β-d-Glucosidases (EC 3.2.1.21) are classical glycoside hydrolases that catalyse the hydrolysis of the nonreducing terminal glucose from β-linked d-gluco-oligosaccharides and aryl-β-d-glucosides. Here, the three-dimensional structures of two industrially important family GH3 β-d-glucosidases from Aspergillus fumigatus and A. oryzae, solved by molecular replacement and refined at 1.95 Å resolution, are reported. Both enzymes, which share 78% sequence identity, display a three-domain structure with the catalytic domain at the interface, as originally shown for barley β-d-glucan exohydrolase, the first three-dimensional structure solved from glycoside hydrolase family GH3.

In AoβG the four protomers in the asymmetric unit are arranged as two dimers, with the second (chains C and D) at right angles to the first (chains A and B), interacting via their FnIII domains (chain A with C and chain B with D). There are no sugar-mediated interactions in the FnIII dimer–dimer interfaces, which are comprised solely of protein–protein and protein–solvent hydrogen bonds, whilst there are a couple of interactions between glycans at the subunit–subunit interface between chains A and B and chains C and D within each dimer, as detailed below. In AoβG there is a PEG molecule bound in the +1 site, hydrogen-bonded to Asp93 OD2 (in three of the four molecules) and/or to Arg99 NH1 (in two of the four protomers in the asymmetric unit). Substrate-specificity studies with AoβG have demonstrated a tight specificity for β-d-glucopyranoside in the −1 subsite, with a much broader tolerance at the +1 subsite with similar catalytic efficiencies for glucose-β-1,2-, β-1,3-, β-1,4- and β-1,6-linked glucose and p-nitrophenyl-β-d-glucopyranoside. There are 13 potential N-glycosylation sites in the amino-acid sequences of each of AfβG and AoβG, with nine and ten of them being occupied in their respective crystal structures; we have modelled 45 and 46 sugars in chains A and B, respectively, for AfβG, whilst AoβG has 40, 42, 41 and 34 sugars modelled in chains A, B, C and D, respectively. The largest N-glycan is linked to Asn323 in domain A, where it is visible as a complete nine-mannose tree in AfβG and AoβG (chains A and B in the latter, chains C and D having seven and six mannoses, respectively). Intriguingly, those sites located on the protein surface (Asn543 and Asn715 in AfβG, Asn212 and Asn543 in AoβG) appear to have been truncated to a single GlcNAc molecule linked to their corresponding Asn residue, despite no attempt having been made to remove external N-glycans enzymatically. In addition, the external site at Asn713 in AoβG (equivalent to Asn715 in AfβG) remained uncleaved even though the first GlcNAc molecule is in a very similar position and orientation to its equivalents in the other two structures.

>[4x]KDDLAYSPPFYPSPWADGQGEWAEVYKRAVDIVSQMTLTEKVNLTTGTGWQLERCVGQTGSVPRLNIPSLCLQDSPLGIRFSDYNSAFPAGVNVAATWDKTLAYLRGQAMGEEFSDKGIDVQLGPAAGPLGAHPDGGRNWEGFSPDPALTGVLFAETIKGIQDAGVIATAKHYIMNEQEHFRQQPEAAGYGFNVSDSLSSNVDDKTMHELYLWPFADAVRAGVGAVMCSYNQINNSYGCENSETLNKLLKAELGFQGFVMSDWTAHHSGVGAALAGLDMSMPGDVTFDSGTSFWGANLTVGVLNGTIPQWRVDDMAVRIMAAYYKVGRDTKYTPPNFSSWTRDEYGFAHNHVSEGAYERVNEFVDVQRDHADLIRRIGAQSTVLLKNKGALPLSRKEKLVALLGEDAGSNSWGANGCDDRGCDNGTLAMAWGSGTANFPYLVTPEQAIQNEVLQGRGNVFAVTDSWALDKIAAAARQASVSLVFVNSDSGEGYLSVDGNEGDRNNITLWKNGDNVVKTAANNCNNTVVIIHSVGPVLIDEWYDHPNVTGILWAGLPGQESGNSIADVLYGRVNPGAKSPFTWGKTRESYGSPLVKDANNGNGAPQSDFTQGVFIDYRHFDKFNETPIYEFGYGLSYTTFELSDLHVQPLNASRYTPTSGMTEAAKNFGEIGDASEYVYPEGLERIHEFIYPWINSTDLKASSDDSNYGWEDSKYIPEGATDGSAQPRLPASGGAGGNPGLYEDLFRVSVKVKNTGNVAGDEVPQLYVSLGGPNEPKVVLRKFERIHLAPSQEAVWTTTLTRRDLANWDVSAQDWTVTPYPKTIYVGNSSRKLPLQASLPKAQ>[2x]GNTTSSVILTNYMDTQYYGEIGIGTPPQTFKVVFDTGSSNVWVPSSKCSRLYTACVYHKLFDASDSSSYKHNGTELTLRYSTGTVSGFLSQDIITVGGITVTQMFGEVTEMPALPFMLAEFDGVVGMGFIEQAIGRVTPIFDNIISQGVLKEDVFSFYYNR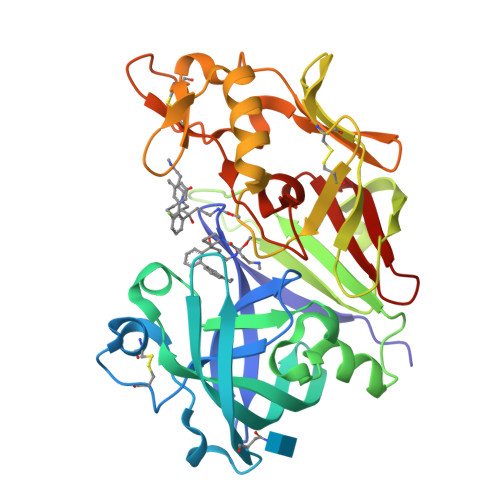DSENSQSLGGQIVLGGSDPQHYEGNFHYINLIKTGVWQIQMKGVSVGSSTLLCEDGCLALVDTGASYISGSTSSIEKLMEALGAKKRLFDYVVKCNEGPTLPDISFHLGGKEYTLTSADYVFQESYSSKKLCTLAIHAMDIPPPTGPTWALGATFIRKFYTEFDRRNNRIGFALAR>SMSRPDQAARRRAIAAELHVSPTFDARDEAERRIGFVADYLRTAGLRACVLGISGGIDSSTAGRLAQLAVERLRASGYDARFVAMRLPYGAQHDEADARRALAFVRADETLTVDVKPAADAMLAALAAGGLAYLDHAQQDFVLGNIKARERMIAQYAVAGARNGVVIGTDHAAESVMGFFTKFGDGGADVLPLAGLTKRRVRALARMLGADEPLVLKTPTADLETLRPQRPDEHAYGITYEQIDDFLEGKPMDDAVAETVLRFYDATRHKRALPYT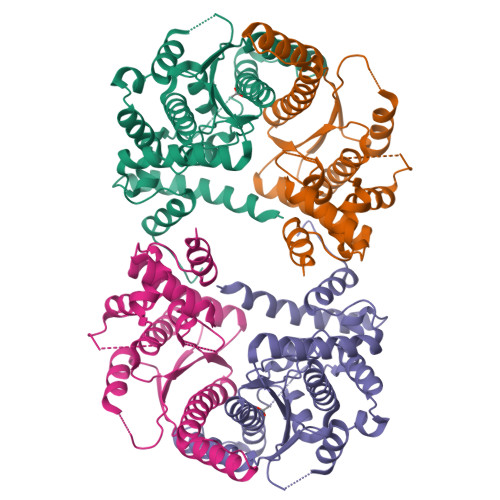MFDWPGHPA[2x]> SMPQALSTDILIVGGGIAGLWLNARLRRAGYATVLVESASLGGGQSVKSQGIIHGGAKYALHGALTGASEAIADMPRRWRACLGSDGELDLRGVRLLSEAHYLWSPGGLAGSLTSFFASKAVRSRVEQAKGEDLPPALRDKGFKGKAYRLTEIVFDVPDLIRRLAELAGDSLLAGERIEPLREGRELAGLCVDGREIRAQRVVLSAGAGNEALLRELGLEQPAMQRRPLHMVMVKAATLKPLYAHCLGAGPKPRITVTTHPTRDGQSVWYLGGDIAETDGVARDEAAQIAEARRELAKLLPWIDLGQAQWATLRVDRAEPAQSNLLRPDNAFLAEQGRLLVGWPTKLALAPDFADRVCARLEEDGIRPSEHAALPQLPRPPLAEPAWEVAFA

Locus PA4991 had been annotated to encode a flavin-binding protein of 391 amino acids. Analysis of the structure of PA4991 identifies this enzyme as a member of the GR2 family of flavoenzymes. The function of this essential enzyme in the virulence and survival of P. aeruginosa in the host nevertheless remains elusive.

The structure of PA4991 was eventually solved by a combination of molecular replacement using a truncated search model generated from the sequence of PA4991 with Rosetta and phase improvement using a low-occupancy heavy-metal derivative obtained by soaking crystals with phenylmercuric chloride. The refined model of PA4991 consists of one polypeptide chain comprising residues 1–391, one FAD molecule, 41 water molecules and two Hg2+ ions bound on opposite sides of the thiol group of Cys245, albeit with low occupancy. Three loop regions, residues 55–67, 106–125 and 248–249, lacked electron density and appeared to be disordered in the crystal, and therefore were not modelled. FAD is bound noncovalently to PA4991 in an extended conformation in a manner similar to that observed in other members of the GR2 family. The ADP moiety of FAD binds to the classic nucleotide-binding fold, including the diphosphate-binding fingerprint motif GxGxxG, which in PA4991 is represented by the sequence Gly13-Gly14-Gly15-Ile16-Ala17-Gly18 at the end of strand β2 in the central β-sheet of the domain. The isoalloxazine ring is located in an accessible pocket with the re face of FAD facing the solvent. Accessibility of the cofactor in PA4991 appears in part to be controlled by the loop comprising residues 54–67, which is disordered in PA4991. In the vicinity of the isoalloxazine ring there are the side chains of His53, Arg316 and Lys345 that potentially could be involved in ligand binding and/or catalysis. Enzymatic assays did not support a function as a G3P dehydrogenase/oxidase or an amino-acid oxidase as hypothesized based on the three-dimensional structure. The conservation of the active-site arginine residue involved in the binding of negatively charged groups of the substrate in these enzymes suggests that the unknown substrate of PA4991 might also carry a negatively charged phosphate or carboxyl group.6-cyclohexylhexyl beta-D-glucopyranoside 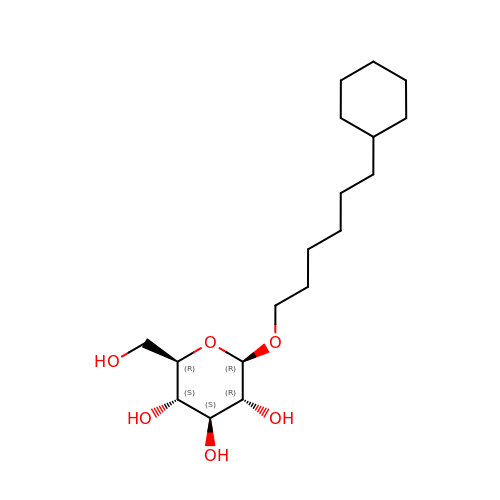| C18 H34 O6 | IKXDBGTYPHAFNV-UYTYNIKBSA-N>[2x]GSGEAD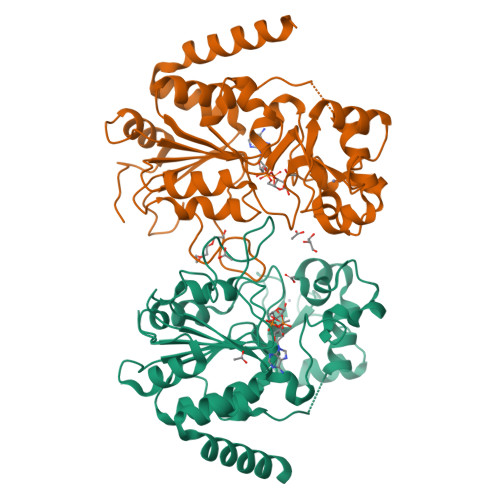MDFLRNLFSQTLSLGSQKERLLDELTLEGVARYMQSERCRRVICLVGAGISTSAGIPDFRSPSTGLYDNLEKYHLPYPEAIFEISYFKKHPEPFFALAKELYPGQFKPTICHYFMRLLKDKGLLLRCYTQNIDTLERIAGLEQEDLVEAHGTFYTSHCVSASCRHEYPLSWMKEKIFSEVTPKCEDCQSLVKPDIVFFGESLPARFFSCMQSDFLKVDLLLVMGTSLQVQPFASLISKAPLSTPRLLINKEKAGQSDPFLGMIMGLGGGMDFDSKKAYRDVAWLGECDQGCLALAELLGWKKELEDLVRREHASIDAQS> MAEKQRQLKLQKIYKQKYIGLGDESTTREQWQRNVRNDTLNTLQG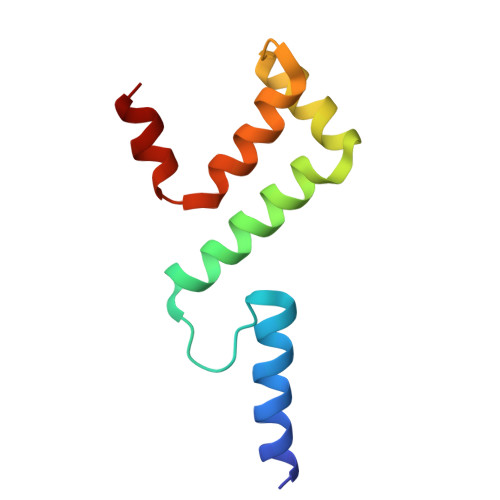HSASLEYVSLSRGDLSIRDTRIHLLKSMSPGYKAYLREE> SMLSSRNRPEGKVLETVGVFEVPKQNGKYETGQLFLHSIFGYRGVVLFPWQARLYDRDVASAAPEKAENPAGHGSKEVKGKTHTYYQVLIDARDCPHISQRSQTEAVTFLANHDDSRALYAIPGLDYVSHEDILPYTSTDQVPIQHELFERFLLYDQTKAPPFVARETLRAWQEKNHPWLELSDVHRETTENIRVTVIPFYMGMREAQN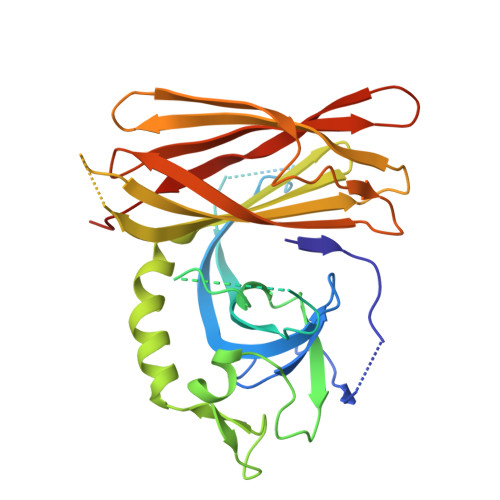SHVYWWRYCIRLENLDSDVVQLRERHWRIFSLSGTLETVRGRGVVGREPVLSKEQPAFQYSSHVSLQASSGHMWGTFRFERPDGSHFDVRIPPFSLESNKDEKTPPSGLHW> MGSSHHHHHHSSGEDRYKEKLLQKAKAEGVESIEELKKRLADQIEEKKKELNKIDPLRELEQHLNAGSRIHTNKEHKTTKMSNKSNEKSGNVLPKDKPYKTLDDYLKLDKIKDLSKQEVEFLWRAKWSNRDDSLVAVVP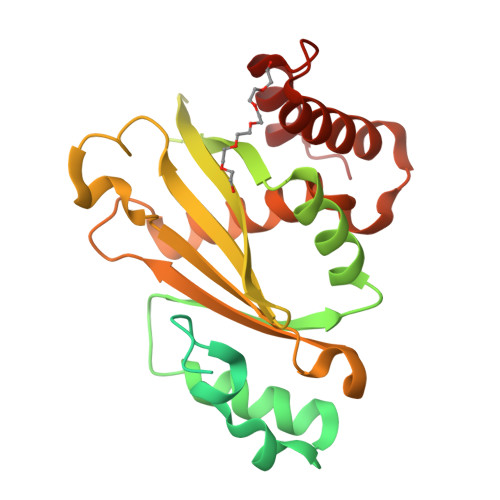YVKTFQGMYKYAVKNPLFVLPLPRENAADGNKADKDSVPVELQYVQWQFAGPNTVHCLITSLAEYKLHQDFAKPHTTIQFHLDLANDKDMVLMNGQVESDSNVSLQDAQLLLLNVQRFYGAMGSETSIAKERIQLLEDFNKGSQNFDINKLIQLAQSMEN> MEDLALRPKTLDEYIGQERLKQKLRVYLEAAKARKEPLEHLLLFGPPGLGKTTLAHVIAHELGVNLRVTSGPAIEKPGDLAAILANSLEEGDILFIDEIHRLSRQAEEHLYPAMEDFVMDIVIGQGPAARTIRLELPRFTLIGATTRPGLITAPLLSRFGIVEHLEYYTPEELAQGVMRDARLLGVRITEEAALEIGRRSRGTMRVAKRLFRRVRDFAQVAGEEVITRERALEALAALGLDELGLEKRDREILEVLI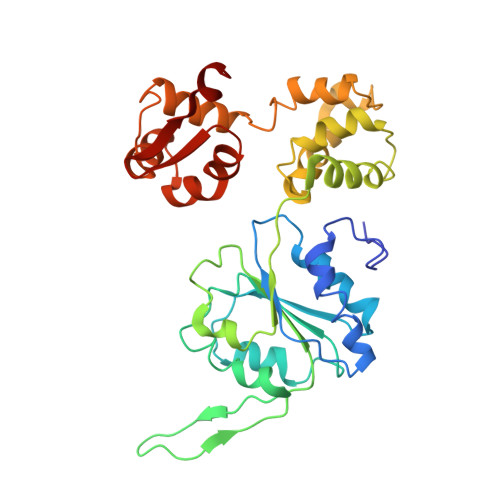LRFGGGPVGLATLATALSEDPGTLEEVHEPYLIRQGLLKRTPRGRVATELARRHL> GSVPATLPQLT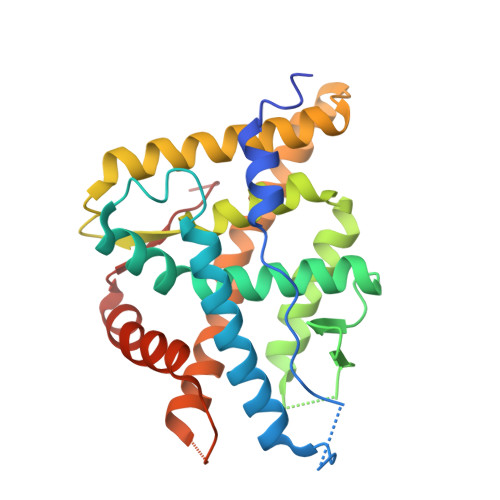PTLVSLLEVIEPEVLYAGYDSSVPDSTWRIMTTLNMLGGRQVIAAVKWAKAIPGFRNLHLDDQMTLLQYSWMYLMAFALGWRSYRQSSANLLCFAPDLIINEQRMTLPGMYDQCKHMLYVSSELHRLQVSYEEYLCMKTLLLLSSVPKDGLKSQELFDEIRMTYIKELGKAIVKREGNSSQNWQRFYQLTKLLDSMHEVVENLLNYCFQTFLDKTMSIEFPEMLAEIITNQIPKYSNGNIKKLLFHQK>[2x]MAHHHHHHVFFAVITLFPEMFDAITAYGISGRAAKRDIVQVTCINPRDFAEGNYRRVDERPFGGGPGMVMMAEPLAKAINHAKQLASRAGCVHVPVVYMSPQGKTLNEQAVQQFVDY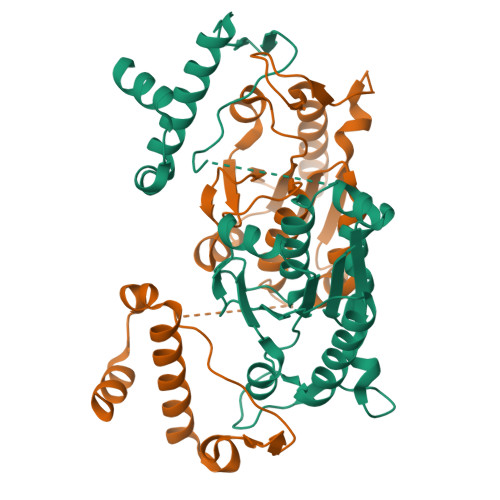DGLIVLCGRYEGVDERLIQHYVDQEWSIGDYVLSGGELPAMVLLDSIIRRLPNVMSDEQSAIQDSFVDGLLDCPQYTKPDQFEGLDVPEILKSGHHANIEKWRFLQRYQRTLERRPELIEQVTLTKQQKKWLSDEQG>[6x]MSGGRAPAVLLGGVASLLLSFVWMPALLPVASRLLLLPRVLLTMASGSPPTQPSPASDSG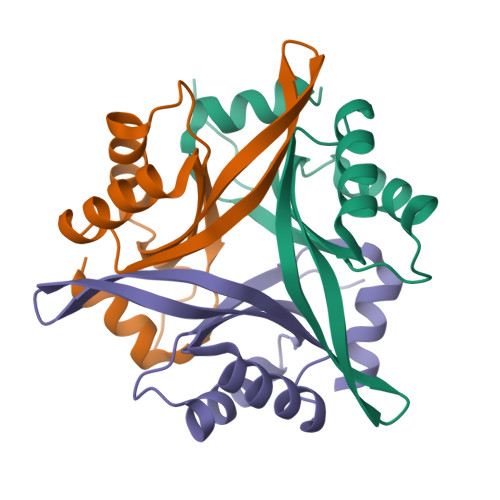SGYVPGSVSAAFVTCPNEKVAKEIARAVVEKRLAACVNLIPQITSIYEWKGKIEEDSEVLMMIKTQSSLVPALTDFVRSVHPYEVAEVIALPVEQGNFPYLQWVRQVTESVSDSITVLP>MRVIVFFDLPVITPENRHNYSVFRKYLIKSGFIMQQKSVYSKLVLNLTNRDSIVKSIEKNKPPE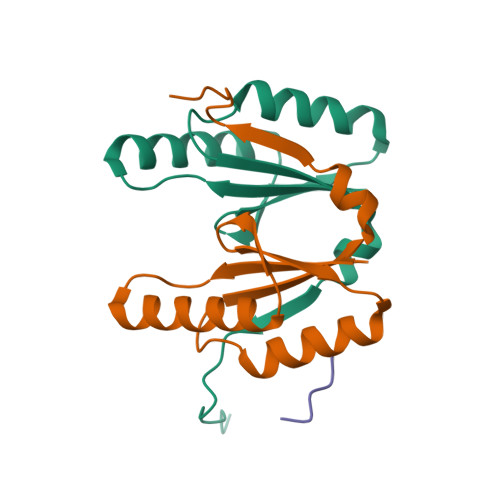GLVEVLTVTEKQYAKMEIIIGESKTEYLNTDERLVVL[2x];> IELSG> MSSVSIFGLGAMGTALASRFLEEKYKVAVWNRSPEKASSLLGKGATLSHTAVDGINASDLIIICLLDNAAVEATLAGALDHLHGKTIINLTNGTPDQARKLSDRFVSHGARYVHGGIMATPSMIGSPYALVLYSGSPDAFKAAEGDLSVLAKCVFLGEDAGTASLHD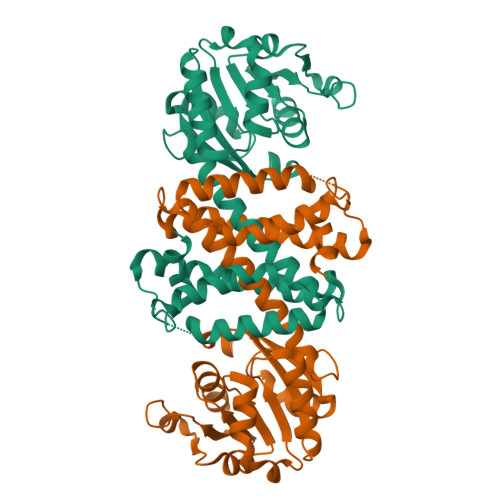LALLSGMYGLFSGFLHATALVRSSTPAVKFMDLLVPWLGAMTEYTKGMAKQIDEGKYTSEGSNLAMQLVGIQNIIDASEAQQVSAEFIRPMKEFMQKAVAAGHGGDDISSLIDFVKST> SGISLDNSYKMDYPEMGLCIIINNKNFHKSTGMTSRSGTDVDAANLRETFRNLKYEVRNKNDLTREEIVELMRDVSKEDHSKRSSFVCVLLSHGEEGIIFGTNGPVDLKKITNFFRGDRCRSLTGKPKLFIIQACRGTELDCGIETDSGVDDDMACHKIPVEADFLYAYSTAPGYYSWRNSKDGSWFIQSLCAMLKQYADKLEFMHILTRVNRKVAT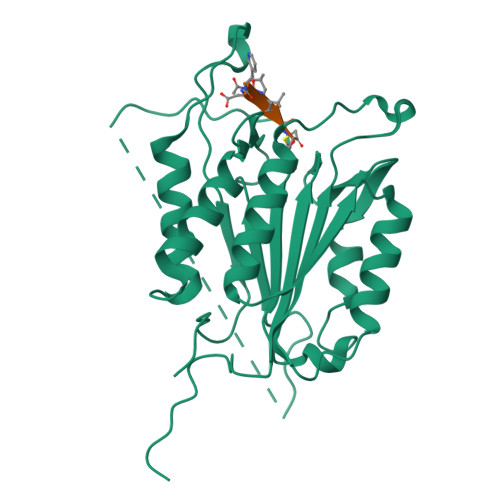EFESFSFDATFHAKKQIPCIVSMLTKELYFYHQLHHHHHH> GSHMDYILGRYVKIARYGSGGLVGGGGKEQYVENLVLWENIIKTAYCFITPSSYTAALETANIPEKDFSNCFRFLKENFFIIPGEYNNSTENNRYSRNFLHYQSYGANPVLVQDKLKNAKVVILGCGGIGNHVSVILATSGIGEIILIDNDQIENTNLTRQVLFSEDDVGKNKTEVIKRELLKRNSEISVSEIALNINDYTDLHKVPEADIWVVSADHPFNLINWVNKYCVRANQPYINAGYVNDIAVFGPLYVPGKTGCYECQKVVADLYGSEKENIDHKIKLINSRFKPATFAP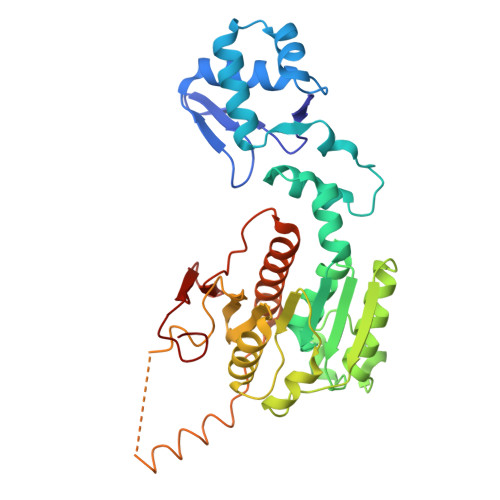VNNVAAALCAADVIKFIGKYSEPLSLNKRIGIWSDEIKIHSQNMGRSPVCSVCGNRM>MAKVSLEKDKIKFLLVEGVHQKALESLRAAGYTNIEFHKGALDDEQLKESIRDAHFIGLRSRTHLTEDVINAAEKLVAIGCFCIGTNQVDLDAAAKRGIPVFNAPFSNTRSVAELVIGELLLLLRGVPEANAKAHRGVWNKLAAGSFEARGKKLGIIGYGHIGTQLGILAESLGMYVYFYDIENKLPLGNATQVQHLSDLLNMSDVVSLHVPENPSTKNMMGAKEISLMKPGSLLINASRGTVVDIPALCDALASKHLAGAAIDVFPTEPATNSDPFTSPLCEFDNVLLTPHIGGSTQEAQENIGLEVAGKLIKYSDNGSTLSAVNFPEVSLPLHGGRRLMHIHENRPGVLTALNKIFAEQGVNIAAQYLQTSAQMGYVVIDIEADEDVAEKALQA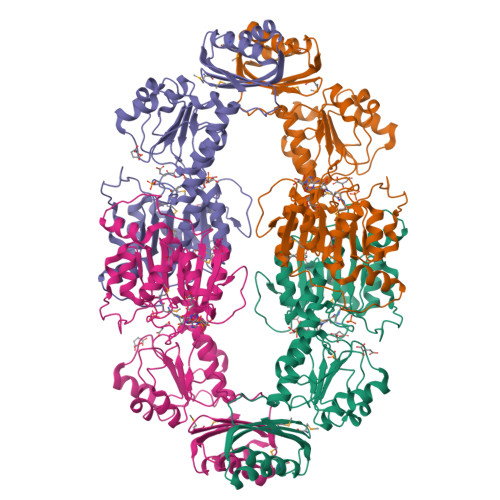MKAIPGTIRARLLY[4x]> MGMSFLGGFFGPICEIDIVLNDGETRKMAEMKTEDGKVEKHYLFYDGESVSGKVNLAFKQPGKRLEHQGIRIEFVGQIELFNDKSNTHEFVNLVKELALPGELTQSRSYDFEFMQVEKPYESYIGANVRLRYFLKVTIVRRLTDLVKEYDLIVHQLATYPDVNNSIKMEVGIEDCLHIEFEYNKSKYHLK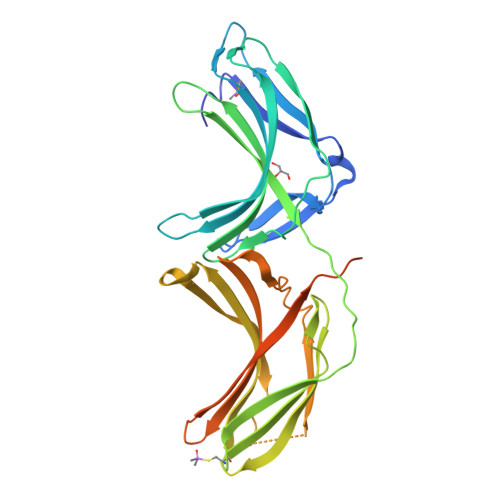DVIVGKIYFLLVRIKIQHMELQLIKKEITGIGPSTTTETETIAKYEIMDGAPVKGESIPIRLFLAGYDPTPTMRDVNKKFSVRYFLNLVLVDEEDRRYFKQQEIILWRKAPEKLRKQRTNFHQRFESPESQASAEQPEMGLVPRGSHHHHH>GSHLDPRKARDIPDEHYQRIIETRDAIQNKYSK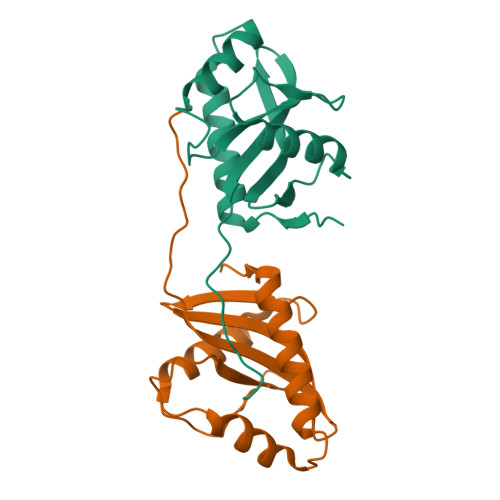ETDLGRILFRVEGNRAGKHDPRPRVFFSDYNGNVLTTDKRSNFQLRAMQNFVTSIEDYNKPKQRLYGRYMIAGPVPIVLADSELLMYVGFKWNEPPPLLLRLFDH[2x]>MGSSHHHHHHSSPRLFMLSSTSSDALRQTARQLATWVEEHQDCVAASDLAYTLARGRAHRPVRTAVVAANLPELVEGLREVADGDALYDAAVGHGDRGPVWVFSGQGSQWAAMGTQLLASEPVFAATIAKLEPVIAAESGFSVTEAITAQQTVTGIDKVQPAVFAVQVALAATMEQTYGVRPGAVVGHSMGESAAAVVAGALSLEDAARVICRRSKLMTRIAGAGAMGSVELPAKQVNSELMARGIDDVVVSVVASPQSTVIGGTSDTVRDLIARWEQRDVMAREVAVDVAFHSPQV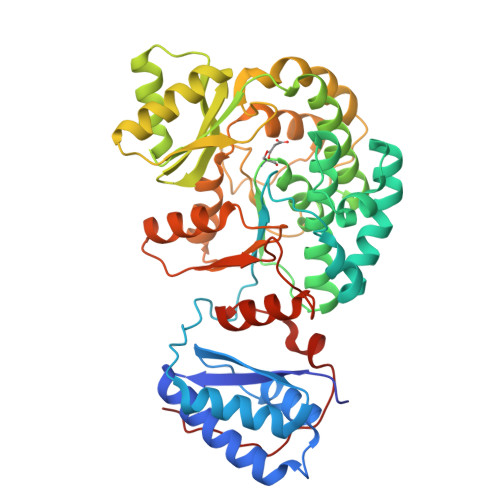DPILDDLAAALADIAPMTPKVPYYSATLFDPREQPVCDGAYWVDNLRNTVQFAAAVQAAMEDGYRVFAELSPHPLLTHAVEQTGRSLDMSVAALAGMRREQPLPHGLRGLLTELHRAGAALDYSALYPAGRLVDAPLPAWGS[2x]>[6x]ARQSQLSPQNQCQLNQLQAREPDNRIQAEAGQIETWNFNQGDFQCAGVAASRITIQRNGLHLPSYSNAPQLIYIVQGRGVLGAVFSGCPETFEESQQSSQQGRQQEQEQERQQQQQGEQGRQQGQQEQQQERQGRQQGRQQQEEGRQQEQQQGQQGRPQQQQQFRQLDRHQKTRRIREGDVVAIPAGVAYWSYNDGDQELVAVNLFHVSSDHNQLDQNPRKFYLAGNPENEFNQQGQSQPRQQGEQGRPGQHQQPFGRPRQQEQQGNGNNVFSGFNTQLLA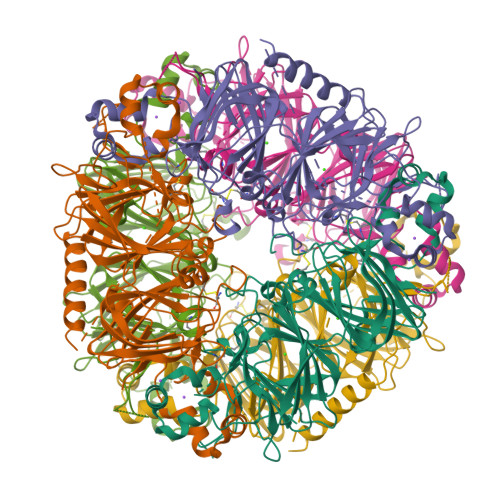QALNVNEETARNLQGQNDNRNQIIQVRGNLDFVQPPRGRQEREHEERQQEQLQQERQQQGEQLMANGLEETFCSLRLKENIGNPERADIFSPRAGRISTLNSHNLPILRFLRLSAERGFFYRNGIYSPHWNVNAHSVVYVIRGNARVQVVNENGDAILDQEVQQGQLFIVPQNHGVIQQAGNQGFEYFAFKTEENAFINTLAGRTSFLRALPDEVLANAYQISREQARQLKYNRQETIALSSSQQRRAVV>HHHHHSRKTYTLTDYLKNTYRLKLYSLRWISDHEYLYKQENNILVFNAEYGNSSVFLENSTFDEFGHSINDYSISPDGQFILLEYNYVKQWRHSYTASYDIYDLNKRQLITEERIPNNTQWVTWSPVGHKLAYVWNNDIYVKIEPNLPSYRITWTGKEDIIYNGITDWVYEEEVFSAYSALWWSPNGTFLAYAQFNDTEVPLIEYSFYSDESLQYPKTVRVPYPKAGAVNPTVKFFVVNTDSLSSVTNATSIQITAPASMLIGDHYLCDVTWATQERISLQWLRRIQNYSVMDICDYDESSGRWNCLVARQHIEMSTTGWVGRFRPSEPHFTLDGNSFYKIISNEEGYRHICYFQIDKKDCTFITKGTWEVIGIEALTSDYLYYISNEYKGMPGGRNLYKIQLSDYTKVTCLSCELNPERCQYYSVS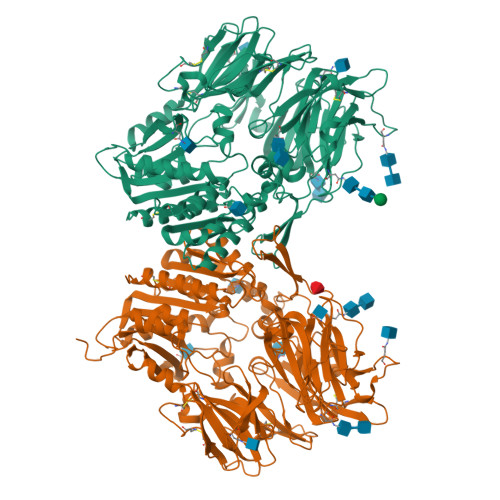FSKEAKYYQLRCSGPGLPLYTLHSSVNDKGLRVLEDNSALDKMLQNVQMPSKKLDFIILNETKFWYQMILPPHFDKSKKYPLLLDVYAGPCSQKADTVFRLNWATYLASTENIIVASFDGRGSGYQGDKIMHAINRRLGTFEVEDQIEAARQFSKMGFVDNKRIAIWGWSYGGYVTSMVLGSGSGVFKCGIAVAPVSRWEYYDSVYTERYMGLPTPEDNLDHYRNSTVMSRAENFKQVEYLLIHGTADDNVHFQQSAQISKALVDVGVDFQAMWYTDEDHGIASSTAHQHIYTHMSHFIKQCFSLP[4x]>[2x]MSLFKIRMPETVAEGTRLALRAFSLVVAVDERGGIGDGRSIPWNVPEDMKFFRDVTTKLRGKNVKPSPAKRNAVVMGRKTWDSIPPKFRPLPGRLNVVLSSTLTTQHLLDGLPDEEKRNLHADSIVAVNGGLEQ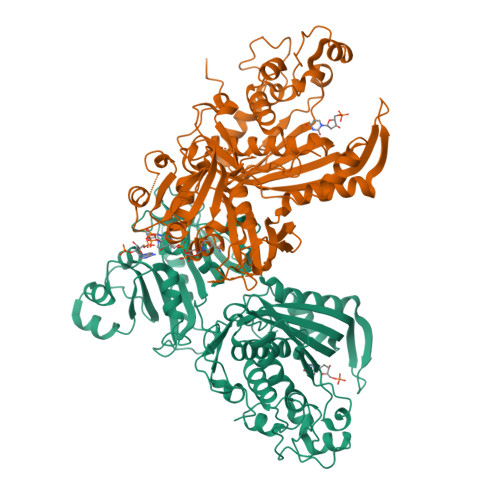ALQLLASPNYTPSIETVYCIGGGSVYAEALRPPCVHLLQAIYRTTIRASESSCSVFFRVPESGTEAAAGIEWQRETISEELTSANGNETKYYFEKLIPRNREEEQYLSLVDRIIREGNVKHDRTGVGTLSIFGAQMRFSLRNNRLPLLTTKRVFWRGVCEELLWFLRGETYAKKLSDKGVHIWDDNGSRAFLDSRGLTEYEEMDLGPVYGFQWRHFGAAYTHHDANYDGQGVDQIKAIVETLKTNPDDRRMLFTAWNPSALPRMALPPCHLLAQFYVSNGELSCMLYQRSCDMGLGVPFNIASYALLTILIAKATGLRPGELVHTLGDAHVYSNHVEPCNEQLKRVPRAFPYLVFRREREFLEDYEEGDMEVIDYAPYPPISMKMAV>[2x]MSRLTGKNALVTGSSRGIGRATAVRLAREGALVAVHYASNEAAADETVAQIERE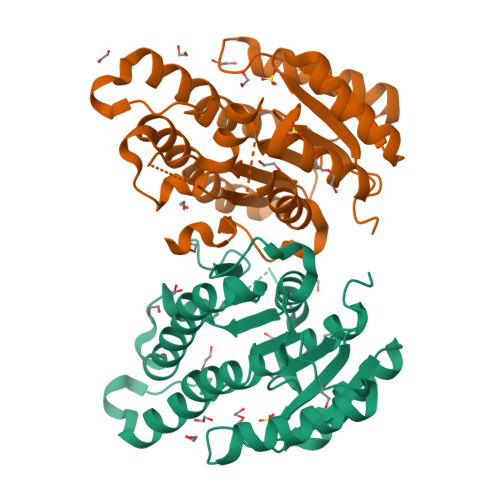GGRAFPVRAELGVAGDVHELFLGLEQGLKERTGETTLDILVNNAAVTGVDGILPEDVTAEQLDRYYAVNAKAPFLLVQRAVRNMPDGGRIINISSGLTRCAVPEQVAYSMTKGALEQITLHMAKHLAPRGITVNSVAPGITDNGGAVFDIPEIVEQMAQSSAFKRVGEAGDVADVVTFIATDESRWITGAFIDASGGTLLG>[2x]MENQKLIANKFNQALGAMQTGFTTTNEAFQKVQD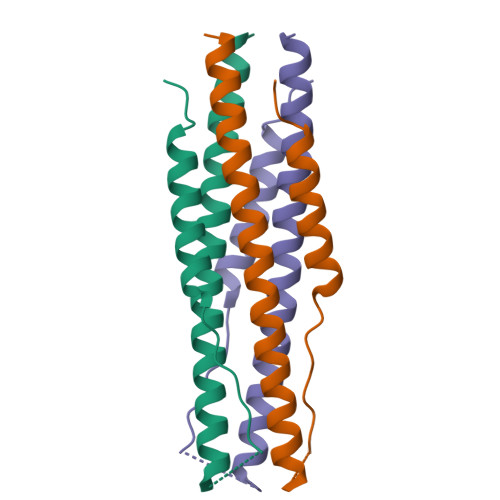AVNNNAQALSKLASELSNTFGAISASIGDILVPRGSGGSGGSGGLEVLFQGPLTQINTTLLDLTYEMLSLQQVVKALNESYIDLKELLEHHHHHH methyl 2-[1-[[3-[3,5-bis(chloranyl)phenyl]-5-[[4-(2-methoxy-2-oxidanylidene-ethyl)piperidin-1-yl]methyl]phenyl]methyl]piperidin-4-yl]ethanoate 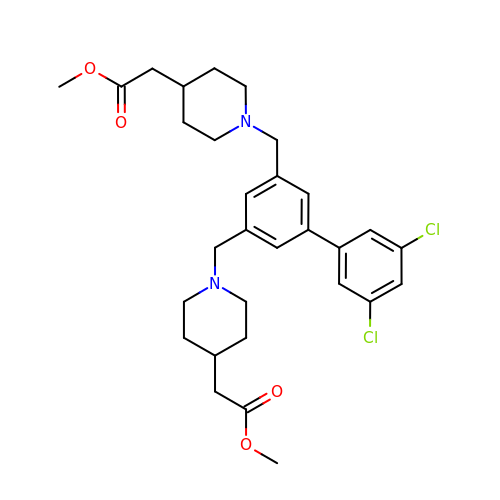| C30 H38 Cl2 N2 O4 | NDWSEVGIFGROAW-UHFFFAOYSA-N> PHLRTFKDNFQTCKVEGAWPLIDNNYLSVQVTNVPVVPGSSATATNKITIIFKAHHGCTDQKVYQAVTDDLPAAFVDGTTSGGDSDAKSLRIVERESGHYVEMHARYIGTTVFVRQ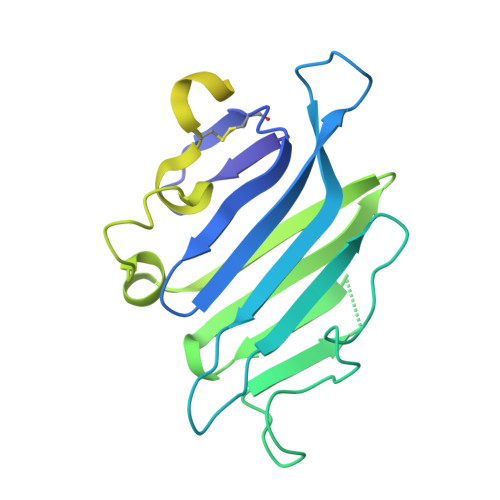VGRYLTLAIRMPEDLAMSYEESQDLQLCVNGCPLSERIDDGQGQVSAILGHSLPRTSLVQAWPGYTLETANTQCHEKMPVKDIYFQSCVFDLLTTGDANFTAAAHSALEDVEALHPRKERWHIFPSGTKHHHHHH(2~{S})-5-azanyl-2-[[[(3~{S})-3-methyl-5-phenyl-pentyl]-oxidanyl-phosphoryl]methyl]-5-oxidanylidene-pentanoic 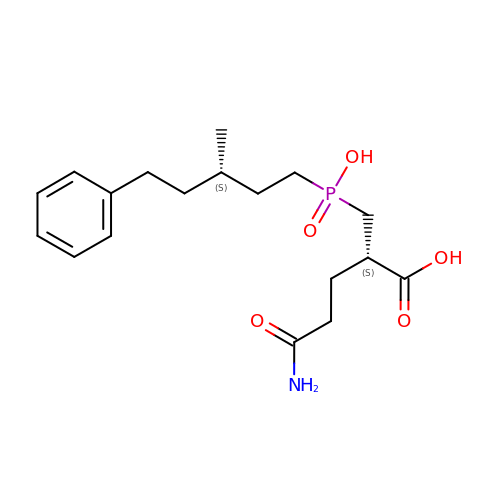acid | C18 H28 N O5 P | QVWDMOWNQBVUFQ-GOEBONIOSA-N>MIEAILFDVDGTLAETEELHRRAFNETFAALGVDWFWDREEYRELLTTTGGKERIARFLRHQKGDPAPLPIADIHRAKTERFVALMAEGEIALRPGIADLIAEAKRAGIRLAVATTTSLPNVEALCRACFGHPAREIFDVIAAGDMVAEKKPSPDIYRLALRELDVPPERAVALEDSLNG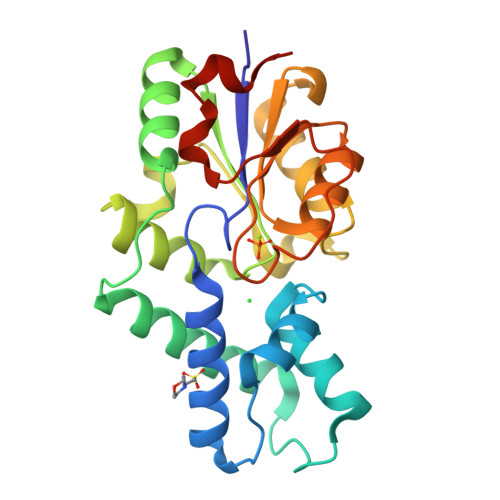LRAAKGAGLRCIVSPGFYTRHEEFAGADRLLDSFAELGGLAGLDLTAPVA[2x]> S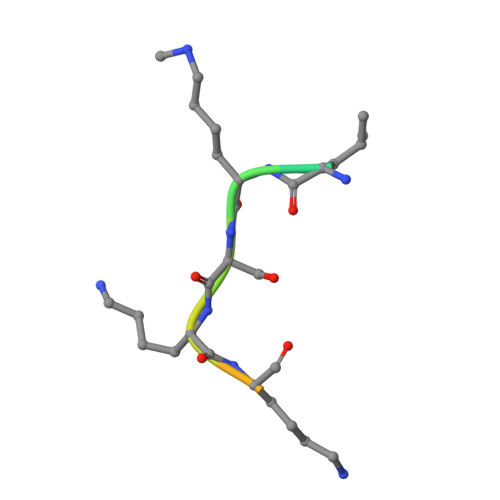SHLKSKKGQSTS> PGYTFTSITLKPPKIDRGSYYGKRLLLPDSVTEYDKKLVSRLQIRVNPLPKFDSTVWVTVRKVPASSDLSVAAISAMFADGASPVLVYQYAASGVQANNKLLYDLSAMRADIGDMRKYAVLVYSKDDALETDELVLHVDIEHQRIPTSGVLPV;> DANFRVLSQQLSRLNKTLAAGRPTINHPTFVGSERCRPGYTFTSITLKPPKIDRGSYYGKRLLLPDSVTEYDKKLVSRLQIRVNPLPKFDSTVWVTVRKVPASSDLSVAAISAMFADGASPVLVYQYAASGVQANNKLLYDLSAMRADIGDMRKYAVLVYSKDDALETDELVLHVDIEHQRIPTSGVLPV;> ADANFRVLSQQLSRLNKTLAAGRPTINHPTFVGSERCRPGYTFTSITLKPPKIDRGSYYGKRLLLPDSVTEYDKKLVSRLQIRVN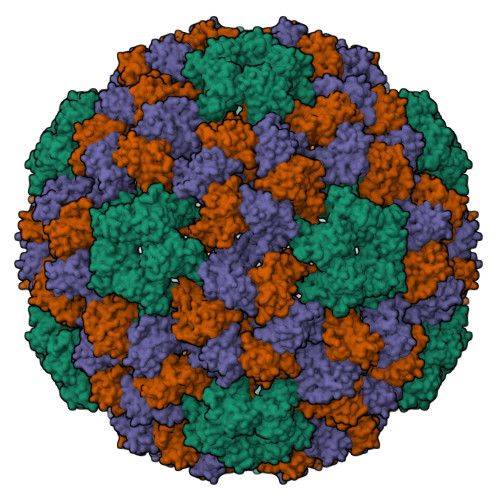PLPKFDSTVWVTVRKVPASSDLSVAAISAMFADGASPVLVYQYAASGVQANNKLLYDLSAMRADIGDMRKYAVLVYSKDDALETDELVLHVDIEHQRIPTSGVLPV> AIGPSANLVVTNAAVAADGHSRDAVVVNGGTPGPLITGNKGDQFQLNVINNLTNFTMLKSTSVHWHGFFQKGTNWADGPAFVNQCPIAAGSSFLYDFSTPIQAGTFWYHSHLSTQYCDGDRGPFVVYDPNDPSANLYDVDNLNTVITLTDWYHTAAQNGPAKPGGADATLINGQGRGPSSPSADLAVISVTAGKRYRFRLVSNSCDPNYTFSIDGHQMTIIQVDSINVQPLVVLK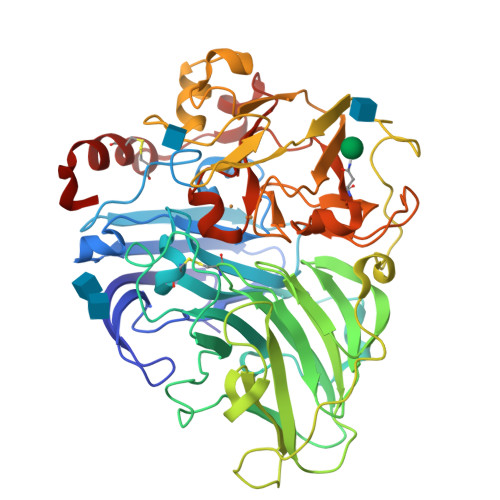IQIYAAQRYSFILNANQAVNNYWIRANPNQGNVGFTNGINSAILRYSGAAATQPTTSQTSSVQPLDQTNLHPLTATAVPGSPVAGGVNLAINQAFNFNGTNHFVDGASFVPPTVPVLSQIVSGAQSAADLLASGLVYSLPSDANIEISFPATSAAAGGPHPFHLHGHAFAVVRSAGSTTYNYNDPIFRDTVSTGTPAANDNVTIRFKTNNPGPWFLHCHIDFHLEAGFAVVFAQDIPDVASANPTPNAWSDLCPVYDAASSSSQ A DNA‐binding protein from starved cells (Dps) protein from nonheterocystous filamentous cyanobacterium Thermoleptolyngbya sp. O‐77 (TlDps1) was purified and characterized. PAGE and CD analyses of TlDps1 illustrated that it had higher thermostability than previously reported Dps proteins.

X‐ray crystallographic analysis revealed that TlDps1 possessed His‐type ferroxidase centers within the cavity and unique metal‐binding sites located on the surface of the protein.

>MAITASPIQTFEQMKDNPIGLEMNVTTAVCEGFNIVLASFQALYLQYQKHHFVVEGSEFYQLHEFFSESYDEVQGHVHEIGERLNGLGGVPVASFSKLAELCCFTPEPDGVFSCRAMVEHDLSAEQEIIKVIRRQAGQAESLGDRATRHLYEKILLESEDRAFHLSHFLAHDSLTPAFTLASQN[6x]> MGSSHHHHHSSGLVPRGSHMASSGFYVDGNTLYDANGQPFVMKGINHGHAWYKDTASTAIPAIAEQGANTIRIVLSDGGQWEKDDIDTVREVIELAEQNKMVAVVEVHDATGRDSRSDLDRAVDYWIEMKDALIGKEDTVIINIANEWYGSWDGAAWADGYIDVIPKLRDAGLTHTLMVDAAGWGQYPQSIHDYGQDVFNADPLKNTIFSIHMYEYAGGDANTVRSNIDRVIDQDLALVIGEFGH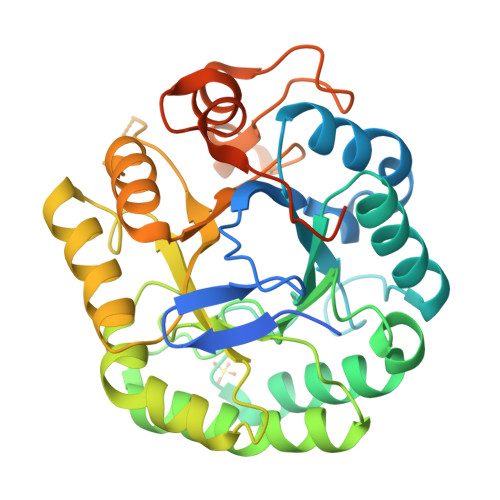RHTDGDVDEDTILSYSEETGTGWLAWSWKGNSAEWDYLDLSEDWAGNHLTDWGNRIVHGANGLQETSKPSTVFTGSEFELRRQACGRTRAPPPPPLRSGC> AQSVPYGVSQIKAPALHSQGYTGSNVKVAVIDSGIDSSHPDLKVAGGASMVPSETNPFQDNNSHGTHVAGTVAALNNSIGVLGVAPSASLYAVKVLGADGSGQYSWIINGIEWAIANNMDVINMSLGGPSGSAALKAAVDKAVASGVVVVAAAGNEGTSGSSSTVGYPGKYPSVIAVGAVDSSNQRASFS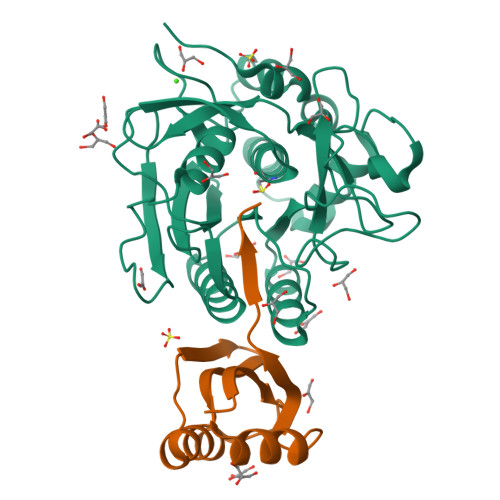SVGPELDVMAPGVSIQSTLPGNKYGAYNGTCMASPHVAGAAALILSKHPNWTNTQVRSSLENTTTKLGDSFYYGKGLINVQAAAQ;> SAGKFIVIFKNDVSEDKIRETKDEVIAEGGTITNEYNMPGMKGFAGELTPQSLTKFQGLQGDLIDSIEEDHVAHAY> MADTDTQKADVVVVGSGVAGAIVAHQLAMAGKAVILLEAGPRMPRWEIVERFRNQPDKMDFMAPYPSSPWAPHPEYGPPNDYLILKGEHKFNSQYIRAVGGTTWHWAASAWRFIPNDFKMKSVYGVGRDWPIQYDDLEPYYQRAEEELGVWGPGPEEDLYSPRKQPYPMPPLPLSFNEQTIKTALNNYDPKFHVVTEPVARNSRPYDGRPTCCGNNNCMPICPIGAMYNGIVHVEKAERAGAKLIENAVVYKLETGPDKRIVAALYKDKTGAEHRVEGKYFVLAANGIETPKILLMSANRDFPNGVANSSDMVGRNLMDHPGTGVSFYASEKLWPGRGPQEMTSLIGFRDGPFRATEAAKKIHLSNLSRIDQETQKIFKAGKLMKPDELDAQIRDRSARYVQFDCFHEILPQPENRIVPSKTATDAIGIPRPEITYAIDDYVKRGAAHTREVYATAAKVLGGTDVVFNDEFAPNNHITGSTIMGADARDSVVDKDCRTFDHPNLFISSS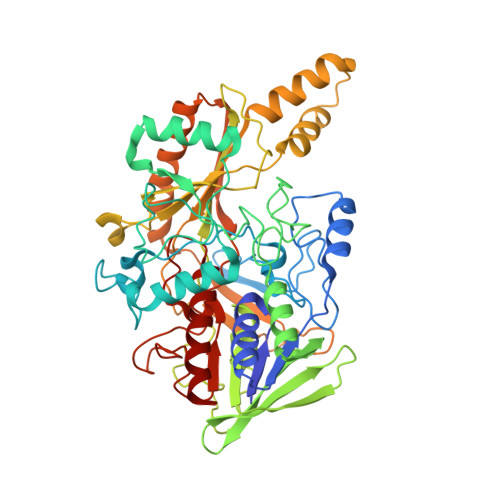ATMPTVGTVNVTLTIAALALRMSDTLKKEV>[3x]MDQDIKTVIQYPVGTTEFDIPFDYLSRKFVRVSLVSDDNRRLLSNITEYRYVSKTRVKLLVATTGFDRVEIRRFTSASERIVDFSDGSVLRANDLNVSQLQSAHIAEEARDAALLAMPEDDAGNLDA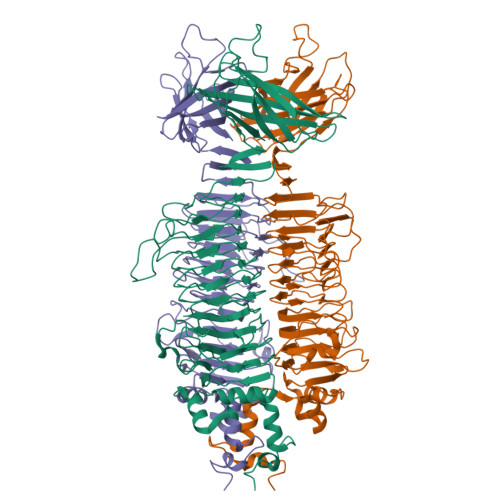RNRKIVRLAPGEAGTDAINKNQLDTTLGEAGGILSEVKDLQKDMEDYLQNWGDDTTAIRGVLWVYNQGSAVGGETSFVITKEGPVLAVPYIEINGSRQYRGWHYEYDLGSKTITLAKPLSAGDLVVCTTAETTLPLADSLAGPTGASQIGTANGLNVQIALDNLRSGVNVLDFMTFAERAAVLNYTGTNDNSEAFRKAFATGSRQIIVPPGRYHVKDVEIPSKVKLFGTYSYKPYNVTSDASFGTDGTIIRKVAGADNMFLWNTACAAEGVMFDGRDRTSPAIQSKSGGKISVGFFKCGFYRFDRVGNRRGAYIGCSFQFCNFNQNNIGIYNTVDGNHIGCTINANKSHGVMLETGANSNTFTNCRNEWNEGDNWNFYGATSIQVINELCDRAFGYGFRISNSSVTLINVNIRRSARTAASGAASAQIYFESSTLKMIGVNSSVGGDDTGGSITEPSPDYFFRMAGTSEGRLEISDSRLTGYTVGLISGTARPSVIRVINSPGWEDTINEGVARISGGRPYIGTMPTATGPANVSPAVLGLSCGGVNTYDNDMFDIHLTIRNTNNGGHNGAILTVLLYREGGAARATIVRVDSRSNAVGEGDVNSTSADPQQVYQVSVEVTSNDASTFNLLVSTKSDNSASYRFRAKVKP>GPLGSLNDIEEIRFTARSEENLRGVHPDLVRVIRLALRYSLVPFSVSEGLRSMARQREMVRAGSSQTLRSRHLTGHAVDVVAMPAGVVSWEWDYYAQIAVAVRRAARECGIIVEWGGEWKTLKDGPHF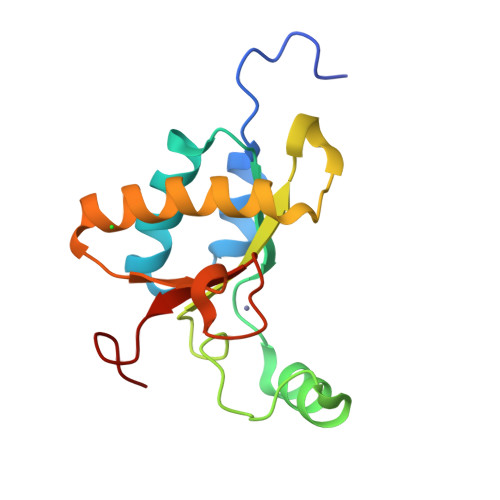QLTFRDYPA[2x]> MPTITPNKLTLKIGRAEGRPGDTVEIPVNLYGVPQKGIASGDFVVSYDPNVLEIIEIEPGELIV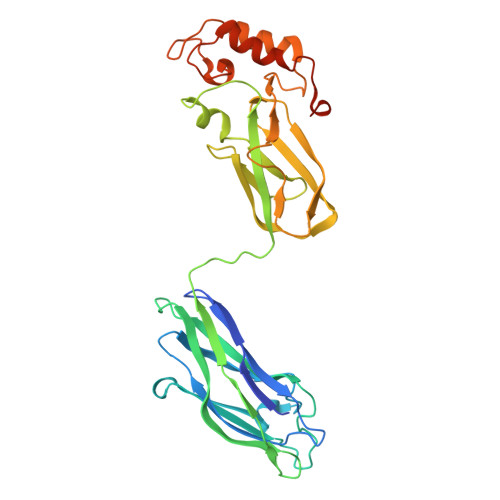DPNPTKSFDTAVYPDRKMIVFLFAEDSGTGAYAITEDGVFATIVAKVKEGAPEGFSAIEISEFGAFADNDLVEVETDLINGGVLVTNKPVIEGYKVSGYILPDFSFDATVAPLVKAGFKVEIVGTELYAVTDANGYFEITGVPANASGYTLKISRATYLDRVIANVVVTGDTSVSTSQAPIMMWVGDIVKDNSINLLDVAEVIRCFNATKGSANYVEELDINRNGAINMQDIMIVHKHFGATSSDYDAQLEHHHHHH> GHMAGNPPDPNAASTGTNPSPQAAGDISPEMMPETANIKLGYIPIVEAAPLIIAQEKGFFAKYGMTGVEVSKQANWASARDNVTIGSQGGGIDGGQWQMPMPHLITEGIITNGNKVPMYVLAQLITQGNGIAVAPMHEGKGVNLDITKAADYIKGFNKTNGRKFKAAHTFPNVNQDFWIRYWFAAGGVDPDTDIDLLAVPPAETVQGMRNGTMDAFSTGDPWPYRIVTENIGYMAGLTAQIWPYHPEEYLAIRADWVDKNPKATKALLKGIMEAQQWIDDPKNRPEVVQIVSGRNYFNVPTTILESPFKGQYTMGDGQPAIDDFQKGPLYWKDGIGNVSYPYKSHDLWF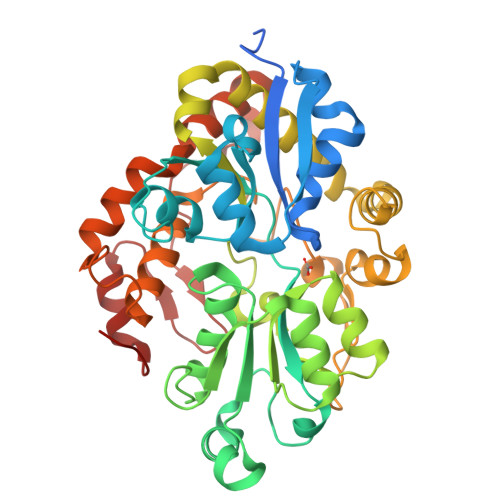LTESIRWGFHKNAIPDLDTAQKIIDKVNREDLWREAATEAGFTADIPSSTSRGVETFFDGITFDPANPSAYLQSLAIKKV>[2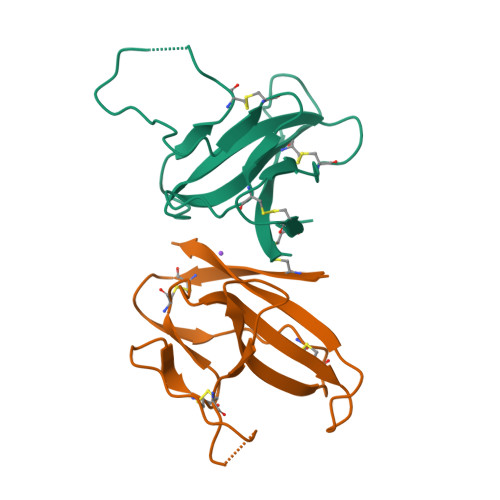x]SNAQECSLQSCTQHQPYVVDDPCPIHFYSKWYIRVGARKSAPLIELCVDEAGSKSPIQYIDIGNYTVSCLPFTINCQEPKLGSLVVRCSFYEDFLEYHDVRVVLDFI> QAPTAVLNGNEVISGVLEGKVDTFKGIPFADPPLNDLRFKHPQPFTGSYQGLKANDFSPACMQLDPGNSLTLLDKAL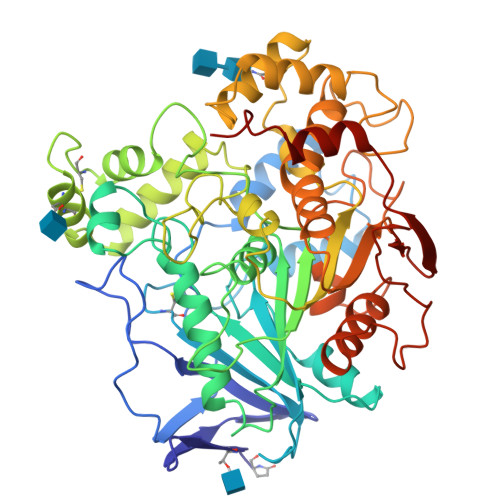GLAKVIPEEFRGPLYDMAKGTVSMNEDCLYLNVFRPAGTKPDAKLPVMVWIYGGAFVYGSSAAYPGNSYVKESINMGQPVVFVSINYRTGPFGFLGGDAITAEGNTNAGLHDQRKGLEWVSDNIANFGGDPDKVMIFGESAGAMSVAHQLIAYGGDNTYNGKKLFHSAILQSGGPLPYHDSSSVGPDISYNRFAQYAGCDTSASANDTLECLRSKSSSVLHDAQNSYDLKDLFGLLPQFLGFGPRPDGNIIPDAAYELFRSGRYAKVPYISGNQEDEGTAFAPVALNATTTPHVKKWLQYIFYDASEASIDRVLSLYPQTLSVGSPFRTGILNALTPQFKRVAAILSDMLFQSPRRVMLSATKDVNRWTYLSTHLHNLVPFLGTFHGNELIFQFNVNIGPANSYLRYFISFANHHDPNVGTNLLQWDQYTDEGKEMLEIHMTDNVMRTDDYRIEGISNFETDVNLYG> REITRTTLQSDQEEIDYDDTISVEMKKEDFDIYDEDENQSPRSFQKKTRHYFIAAVERLWDYGMSSSPHVLRNR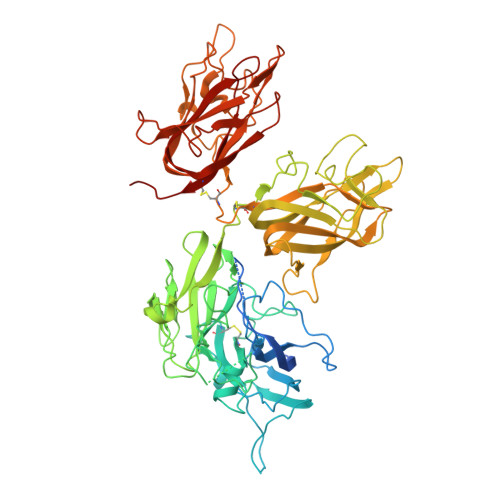AQSGSVPQFKKVVFQEFTDGSFTQPLYRGELNEHLGLLGPYIRAEVEDNIMVTFRNQASRPYSFYSSLISYEEDQRQGAEPRKNFVKPNETKTYFWKVQHHMAPTKDEFDCKAWAYFSDVDLEKDVHSGLIGPLLVCHTNTLNPAHGRQVTVQEFALFFTIFDETKSWYFTENMERNCRAPCNIQMEDPTFKENYRFHAINGYIMDTLPGLVMAQDQRIRWYLLSMGSNENIHSIHFSGHVFTVRKKEEYKMALYNLYPGVFETVEMLPSKAGIWRVECLIGEHLHAGMSTLFLVYSNKCQTPLGMASGHIRDFQITASGQYGQWAPKLARLHYSGSINAWSTKEPFSWIKVDLLAPMIIHGIKTQGARQKFSSLYISQFIIMYSLDGKKWQTYRGNSTGTLMVFFGNVDSSGIKHNIFNPPIIARYIRLHPTHYSIRSTLRMELMGCDLNSCSMPLGMESKAISDAQITASSYFTNMFATWSPSKARLHLQGRSNAWRPQVNNPKEWLQVDFQKTMKVTGVTTQGVKSLLTSMYVKEFLISSSQDGHQWTLFFQNGKVKVFQGNQDSFTPVVNSLDPPLLTRYLRIHPQSWVHQIALRMEVLGCEAQDLY>GDDVMTKEEQIFLLHRAQAQCEKRLKEVLQRPAGRPCLPEWDHILCWPLGAPGEVVAVPCPDYIYD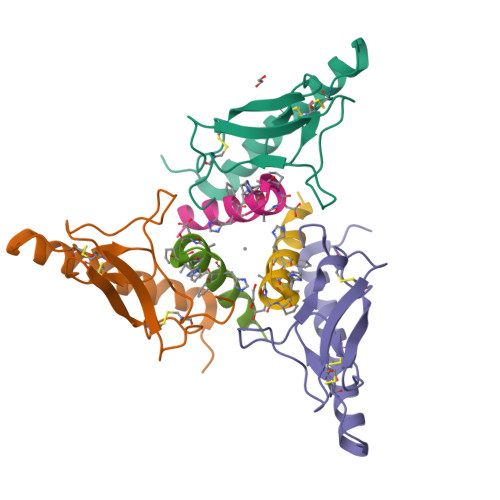FNHKGHAYRRCDRNGSWELVPGHNRTWANYSECVKFL[3x];>YQDLRRRFFXHHLXAEXHTAEI[3x]In mammals, the most abundant and best-studied NDPKs are NME1 and NME2 (hereafter abbreviated NME1/2), which are closely related isoforms (88% sequence identity) with similar functional attributes and localization in the cytosol and nucleus. NME1/2 are hexameric enzymes that catalyze the reaction XTP + YDP ⇆ XDP + YTP by first transferring the γ-phosphoryl group from XTP (usually ATP) to residue His118, and then from the phosphohistidine to YDP, where Y is any of the four common (deoxy)nucleosides. Briefly, each NME1 subunit within the D3-symmetric hexamer comprises an antiparallel four-stranded β sheet flanked on either side by a layer of helices. In this study, we showed that NME1 binds AcCoA and CoA with similar affinity via a binding mode distinct from that of canonical ADP and ATP substrates and critically dependent on the CoA 3′ phosphate group.

Efforts to cocrystallize murine NME1 with the ligands led to high-resolution (1.96 and 2.2 Å, respectively) crystal structures of NME1 bound to SucCoA and ADP, and a somewhat lower (2.6 Å)–resolution structure bound to CoA. ADP is sandwiched between the αA-α2 helical hairpin and an α3-β4 loop segment called the “Kpn loop” that define the enzyme’s active site. Unexpectedly, NME1 recognizes ADP and CoA via completely distinct binding modes. Of the 10 direct hydrogen bonds mediating the NME1:ADP interaction, only two are conserved in the NME1:CoA complex. This is notable because the ligand-interacting residues of NME1 adopt nearly identical conformations in both complexes and because, apart from its 3′ phosphate group, the CoA nucleotide is otherwise chemically identical to ADP. The CoA 3′ phosphate group forms direct H bonds with Lys12, Tyr52, Asn115, and His118 as well as water-mediated H bonds with Arg88, Arg105, and the Gly119 backbone. In the ADP-bound structure, these residues either hydrogen bond with the ribose 2′ and 3’ OH groups or with a water molecule H-bonded to the β phosphate. Similarly, the outward shift of the CoA β phosphate is accommodated by water molecules that satisfy the H bonding potential of residues Arg88 and Arg105, which, in the ADP-bound structure, directly contact the β-phosphate. Compared to ADP, the α and β phosphates of CoA are displaced upward and are solvent accessible, pointing out of the pocket to direct the CoA pantetheine end away from the protein surface. This contrasts with the ADP-bound structure, where the β phosphate is buried deep inside the protein and folds back toward the ribose 3′ OH group, with which it forms an intramolecular H bond critical for catalysis.

>[6x]GAMAMANSERTFIAIKPDGVQRGLVGEIIKRFEQKGFRLVGLKFLQASEDLLKEHYTDLKDRPFFTGLVKYMHSGPVVAMVWEGLNVVKTGRVMLGETNPADSKPGTIRGDFCIQVGRNIIHGSDSVKSAEKEISLWFQPEELVEYKSCAQNWIYE> MGSSHHHHHHSQDPMFDIKRKTIEWGGKTLVLETGRIARQADGAVLATMGETVVLATAVFAKSQKPGQDFFPLTVNYQEKTFAAGKIPGGFFKREGRPSEKETLVSRLIDRPIRPLFVKGFKNEVQVVVTVLQHDLENDPDILGMVAASAALCLSGAPFMGPIGAARVGWVDGAYVLNPTLDEMKESKMDLVVAGTADAVMMVESEIQELSEEIVLGGVNFAHQQMQAVIDAIIDLAEHAAKEPFAFEPEDTDAIKAKMKDLVGADIAAAYKIQKKQDRYEAVGAAKKKAIAALGLSDENPTGYDPLKLGAIFKELEADVVRRGILDTGLRIDGRDVKTVRPILGEVGILPRTHGSALFTRGETQAIVVATLGTGDDEQFIDALEGTYKESFLLHYNFPPYSVGETGRMGSPGRREIGHGKLAWRALRPMLPTKEDFPYTIRLVSEITESNGSSSMATVCGSSLAMMDAGVPLVR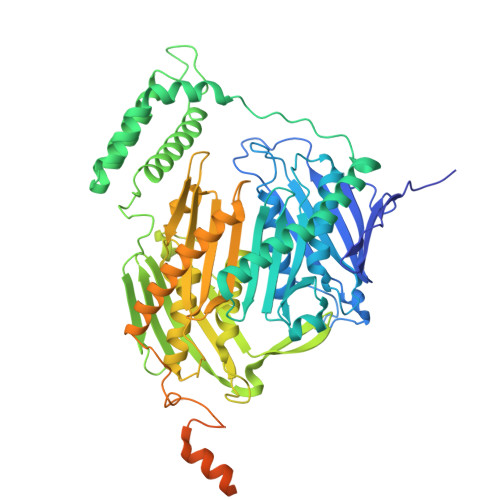PVSGIAMGLILEQDGFAVLSDILGDEDHLGDMDFKVAGTSEGLTSLQMDIKIAGITPAIMEQALAQAKEGRAHILGEMNKAMDAPRADVGDFAPKIETINIPTDKIREVIGSGGKVIREIVATTGAKVDINDDGVVKVSASDGAKIKAAIDWIKSITDEAEVGKIYDGKVVKVVDFGAFVNFFGAKDGLVHVSQISNERVAKPSDVLKEGQMVKVKLLGFDDRGKTKLSMKVVDQETGEDLSKKEAAAEEA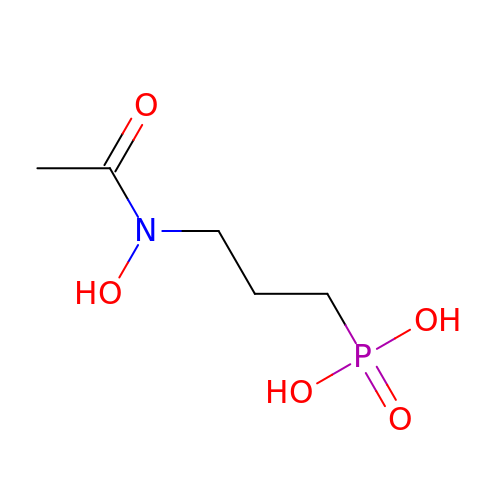3-[ethanoyl(hydroxy)amino]propylphosphonic acid | C5 H12 N O5 P | PKMNDDZSIHLLLI-UHFFFAOYSA-N> TKDLPIHACSYCGIHDPACVVYCNTSKKWFCNGRGNTSGSHIVNHLVRAKCKEVTLHKDGPLGETVLECYNCGCRNVFLLGFIPAKADSVVVLLCRQPCASQSSLKDINWDSSQWQPLIQDRCFLSWLVKIPSEQEQLRARQITAQQINKLEELWKENPSATLEDLEKPGVDEEPQHVLLRYEDAYQYQNIFGPLVKLEADYDKKLKESQTQDNITVRWDLGLNKKRIAYFTLPKTDSDMRLMQGDEICLRYKGDLAPLWKGIGHVIKVPDNYGDEIAIELRSSVGAPVEVTHNFQVDF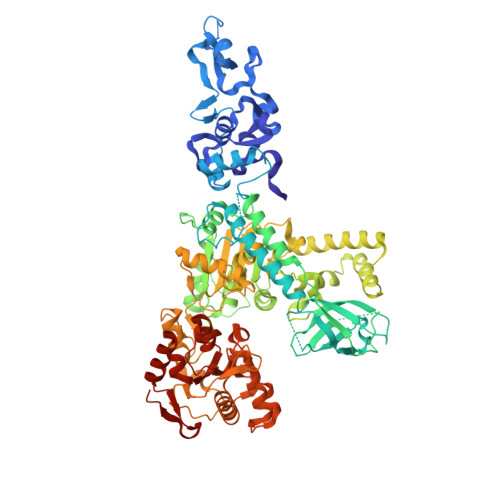VWKSTSFDRMQSALKTFAVDETSVSGYIYHKLLGHEVEDVIIKCQLPKRFTAQGLPDLNHSQVYAVKTVLQRPLSLIQGPPGTGKTVTSATIVYHLARQGNGPVLVCAPSNIAVDQLTEKIHQTGLKVVRLCAKSREAIDSPVSFLALHNQIRNMDSMPELQKLQQLKDETGELSSADEKRYRALKRTAERELLMNADVICCTCVGAGDPRLAKMQFRSILIDESTQATEPECMVPVVLGAKQLILVGDHCQLGPVVMCKKAAKAGLSQSLFERLVVLGIRPIRLQVQYRMHPALSAFPSNIFYEGSLQNGVTAADRVKKGFDFQWPQPDKPMFFYVTQGQEEIASSGTSYLNRTEAANVEKITTKLLKAGAKPDQIGIITPYEGQRSYLVQYMQFSGSLHTKLYQEVEIASVDAFQGREKDFIILSCVRANEHQGIGFLNDPRRLNVALTRARYGVIIVGNPKALSKQPLWNHLLNYYKEQKVLVEGPLNNLRESLMQFS> GPLGSMKQMGSMHPVQVIAVTGGKGGVGKTNVSVNLALALADLGRRVMLLDADLGLANVDVLLGLTPKRTLADVIEGRCELRDVLLLGPGGVRIVPAASGTQSMVHLSPMQHAGLIQAFSDISDNLDVLVVDTAAGIGDSVVSFVRAAQEVLLVVCDEPTSITDAYALIKLLNRDHGMTRFRVLANMAHSPQEGRNLFAKLTKVTDRFLDVALQYVGVIPYDESVRKAVQKQRAVYEAFPRSKASLAFKAVAQKVDSWPLPANPRGHLEFFVE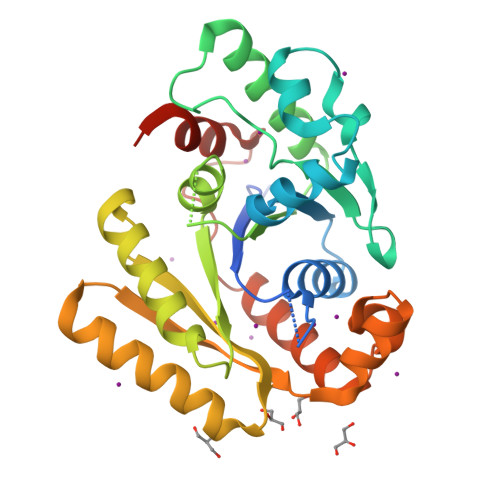RLVQHPATGSAV>[2x]MGMKLLVVSWGDFERWKETKYRFGGETSVGPSTLPILQKVIK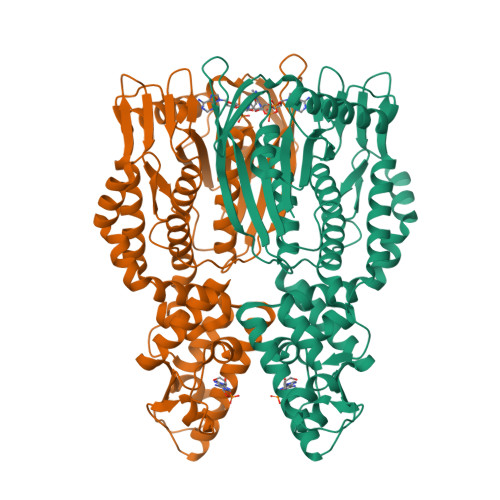PDWTVIVLSDTIGKDFSSVETLREDVRNRVMDFLDRIGAGREVDVIIAPGIGEFTHGSFRGSAMDAYYYVLHALSEIIPTKGDLEVHFDSTHGLNYVTLLTYRALKDLLGIAAVMNTVTFYAYNSDPFVPKITKELNINTIETTMVKPTPLSEPLPGFDEYLCPYSMERAEFVRLKGSLNTLKNLRKEKKKLEAWIGSLLFGLPLLFLEEFPDIGRLESYIEELAETWGGAIAVNAEEKAVTRRLAFGSGFGTLVKLLFQARITRGLLVEEPYSIEKLYSVSDRLFRGSTLQRVRVELGKIEDKAIKYARKGAFPRDIPLRDFLGFDAANREVSPRNVLAHAGLEANVVEVSMEAWEPKRPEEEAGRHTHLKYTPVGLKKVEDIVSRALKESHHHHHH>[3x]MSESFLLNLWILLCACLVLIMQAGFTCFESGNVRNKNSVNVALKNVSDFCVCAVCYWAFGYALMYGNSIDGIVGANGFFYSTTTNSHETSFFLFQLMFCCTSATIISGAVAERMRFTGYILVTLLAASLIYPLFGHWAWGGRILGSETSTPGWLEQLGFIDFAGATVVHSVGGWMALACVLIIGP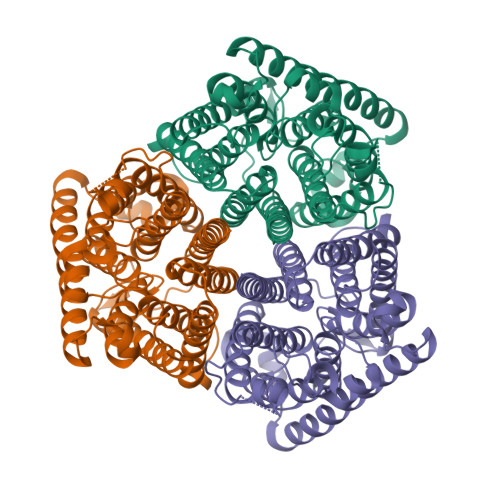RLGRFNNKHGVNQIFGDNLPLTALGTFLLFLGWFGFNGGSYGKIDDMLSSVFVNTALGGTFGGFVVLLICIWQQSLLSIRFVLNGVLAGLVAITASANSISSIDAATIGGISGALSFFATILLEKCKIDDVVSVVPVHLIGGIWGTLALAIFADGQYFIAGNSRVDQFLIQLLGVVTCGIFAFGLPYMLIRLLNRVYPLRVSPRVEILGLNFGEFGLKSETFNFLKQMRKNKNSHKNKQAVSVDFFSDIGLIEAEYNAFLEVINLQQRQADINSHRLSRLAKTDHLTRLNNRLGFDECYDSEWLRMRREKKPFSLLLIDIDHFKLYNDHYGHPRGDQCLQQVALVLASTAKRPADCCARVGGEEFAILLPDTDSEAGEKIANDINIRLKALEIPHLSSPIMPYVTVSIGIATLTPERYDSLDQAYLYQCADDALYSAKQAGRNGVKAVIIDEAHEQTKKLDENLYFQGFEHHHHHH> GSKRDHHQFQGRLSNHGTSSSSSSISKDKMMMVKKEEDGGGNMDDELLAVLGYKVRSSEMAEVALKLEQLETMMSNVQEDGLSHLATDTVHYNPSELYSWLDNMLSELNPPPLPASSNGLDPVLPSPEICGFPASDYDLKVIPGNAIYQFPAIDSSSSSNNQNKRLKSCSSPDSMVTSTSTGTQIGGVIGTTVTTTTTTTTAAGESTRSVILVDSQENGVRLVHALMACAEAIQQNNLTLAEALVKQIGCLAVSQAGAMRKVATYFAEALARRIYRLSPPQNQIDHCLSDTLQMHFYETCPYLKFAHFTANQAILEAFEGKKRVHVIDFSMNQGLQWPALMQALALREGGPPTFRLTGIGPPAPDNSDHLHEVGCKLAQLAEAIHVEFE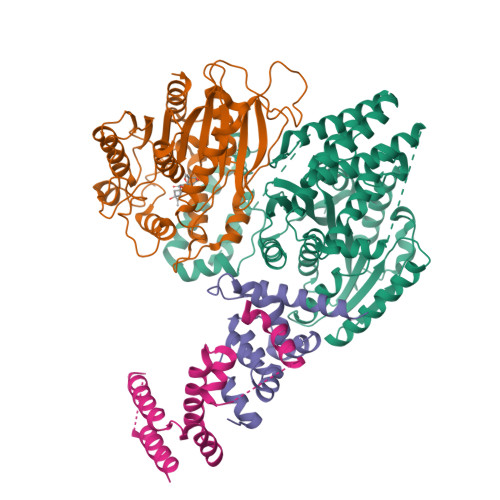YRGFVANSLADLDASMLELRPSDTEAVAVNSVFELHKLLGRPGGIEKVLGVVKQIKPVIFTVVEQESNHNGPVFLDRFTESLHYYSTLFDSLEGVPNSQDKVMSEVYLGKQICNLVACEGPDRVERHETLSQWGNRFGSSGLAPAHLGSNAFKQASMLLSVFNSGQGYRVEESNGCLMLGWHTRPLITTSAWKLSTAAY;> GSMAASDEVNLIESRTVVPLNTWVLISNFKVAYNILRRPDGTFNRHLAEYLDRKVTANANPVDGVFSFDVLIDRRINLLSRVYRPAYADQEQPPSILDLEKPVDGDIVPVILFFHGGSFAHSSANSAIYDTLCRRLVGLCKCVVVSVNYRRAPENPYPCAYDDGWIALNWVNSRSWLKSKKDSKVHIFLAGDSSGGNIAHNVALRAGESGIDVLGNILLNPMFGGNERTESEKSLDGKYFVTVRDRDWYWKAFLPEGEDREHPACNPFSPRGKSLEGVSFPKSLVVVAGLDLIRDWQLAYAEGLKKAGQEVKLMHLEKATVGFYLLPNNNHFHNVMDEISAFVNAEC;> GSMKRSTTDSDLAGDAHNETNKKMKSTEEEEIGFSNLDENLVYEVLKHVDAKTLAMSSCVSKIWHKTAQDERLWELICTRHWTNIGCGQNQLRSVVLALGGFRRLHSLYLWPLSKPNPRARFGKDELKLTLSLLSIRYYEKMSFTKRPLPESK;> GSMSTVRKITLKSSDGENFEIDEAVALESQTIKHMIEDDCTDNGIPLPNVTSKILSKVIEYCKRHVEAAEKSETTADAAAATTTTTVASGSSDEDLKTWDSEFIKVDQGTLFDLILAANYLNIKGLLDLTCQTVADMIKGKTPEEIRKTFNIKNDFTPEEEEEVRRENQWAFE The ‘heat-resistant RNA-dependent ATPase’ Hera is a DEAD box protein from Thermus thermophilus. Hera consists of a helicase core, followed by a bipartite C-terminal extension that contains a dimerization domain (DD) and an RNA-binding domain (RBD). The RBD is responsible for binding of Hera to 23S rRNA fragments comprising hairpin 92 and for binding of RNaseP RNA. The Hera RBD forms a modified RNA recognition motif (RRM).

To visualize the structure of the C-terminal tail of the Hera_RBD, we crystallized several constructs and mutants of Hera_RBD. Two of the mutants, Hera_RBD_K463A and R444A/R449A, yielded structures with their entire C-terminal sequences visible in the electron density maps up to aa 510. In all structures where the C-terminal part is ordered, residues 493-498 fold back onto the outermost β-strand β2 of the RBD and physically block the RNA-binding site (cyan and orange in Figure 5A), with exception of the wild-type Hera_RBD structure. Although the point mutations are likely responsible for the different crystal forms, they do not per se impose this particular conformation of the C-terminus, and only the far ends of the C-termini extending away from the RBD are dictated by crystal contacts. The C-terminal part of the RBD can therefore adopt at least two major orientations, distended from the RBD or attached to the β2 strand. Mutation of K463 abolishes RNA binding (see previously). For the Hera_K463A/32mer and Hera_1-491/32mer complexes, the Kd values were 1.0 ± 0.17 µM and 1.1 ± 0.13 µM. These values are identical to the Kd value of the Hera_core/32mer complex, demonstrating that the RBD does not contribute to RNA binding in these mutants. Mutants were grouped into three classes according to their Kd values: (i) with no or only a moderate (<5-fold) effect on RNA binding (K439A, R487A and R492A), (ii) with an intermediate (5- to 10-fold) effect on RNA binding (R444A and Y472A) and (iii) mutants that showed a >25-fold increase in the Kd values (R449A, R444/449 A, K463A and ΔC-tail).

>[3x]AERSLLTGEEGWRTYKATGPRLSLPRLVALLKGQGLEVGAVAEAEGGFYVDLRPEARPEVAGLRLEPARRVEGLLEIPSRTRRPARA3-({3-[(2-amino-6-fluoropyridin-4-yl)methyl]-5-(1-methylethyl)-2,6-dioxo-1,2,3,6-tetrahydropyrimidin-4-yl}carbonyl)-5-methylbenzonitrile | C22 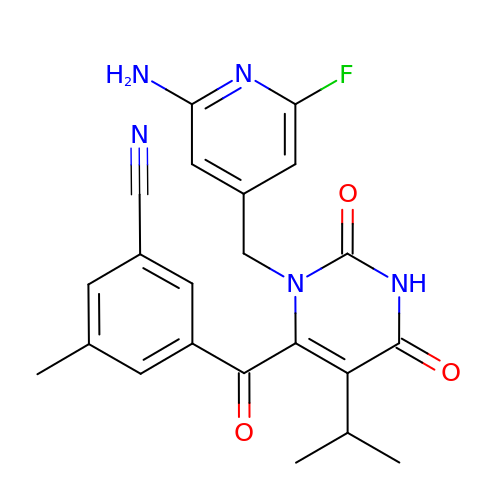H20 F N5 O3 | SORPAQIMHXALKW-UHFFFAOYSA-N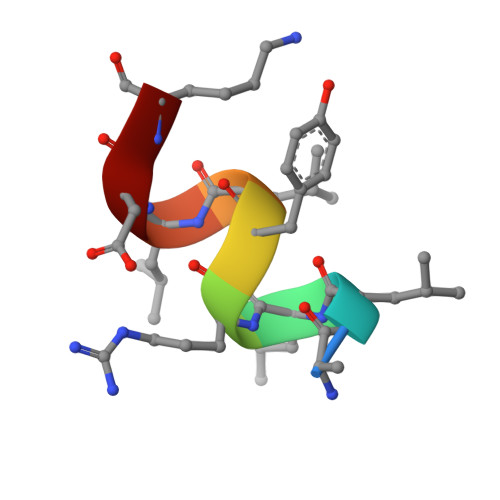> ALLRYLLDK>DAAQPARRAVRSSRHHHHHHGSATCAVYGDGHYLTFDGQSYSFNGDCEYTLVQNHCGGKDSTQDSFRVVTENVPCGTTGTTCSKAIKIFLGGFELKLSHGKVEVIGTDESQEVPYTIQQMGIYLVVDTDIGLVLLWDKKTSIFINLSPEFKGRVCGLCGNFDDIAVNDFATRSRSVVGDVLEFGNSWKLSPSCPDALAPKDPCTANPFRKSWAQKQCSILHGPTFAACHAHVEPARYYEACVNDACACDSGGDCECFCTAVAAYAQACHEVGLCVSWRTPSICPLFCDYYNPEGQCEWHYQPCGVPCLRTCRNPRGDCLRDVRGLEGCYPKCPPEAPIFDEDKMQCVATCPTPPLPPRCHVHGKSYRPGAVVPSDKNCQSCLCTERGVECTYKAEACVCTYNGQRFHPGDVIYHTTDGTGGCISARCGANGTIERRVYPCSPTTPVPPTTFSFSTPPLVVSSTHTPSNGPSSAHTGPPSSAWPTTAGTDDDDKTSEQKLISEEDLSRKLTR[4x]

The two gel-forming mucins MUC5AC and MUC5B constitute the main structural components of the mucus protecting the underlying epithelia in the respiratory system. The VWD assemblies are formed by the VWD domain, C8, trypsin inhibitor like (TIL) and E domains, except the VWD’ domain that only has the TIL and E domains. We determined the cryoEM structures of the wild type D3 assembly of the human MUC5AC mucin and the structural single nucleotide polymorphisms (SNP) variants Arg996Gln and Arg1201Trp that affect intermolecular interactions. The D3 assembly forms covalent dimers that can appear in two alternative conformations, open and closed, where the closed conformation dimers interact through an arginine-rich loop in the TIL3 domain to form tetramers.

Similarly, the structure of the tetrameric 6xHis-MUC5AC-D3 Arg996Gln assembly was solved at low resolution (6–7 Å), not enough to reveal the molecular mechanism of the non-covalent oligomerization. Surprisingly, the 6xHis-MUC5AC-D3 Arg996Gln adopts another conformation not observed in the other variants as the protein forms ring shape octamers. The His-tagged Arg996Gln mutant showed a high proportion of octameric particles in cryoEM that were essential for solving the high-resolution structure of the non-covalent interaction. Particle subtraction followed by local refinement let us solve the structure of a tetramer forming part of the octamer at 3.69 Å resolution. The MUC5AC-D3 non-covalent tetramer interaction is driven by the TIL3 domain and involves an interface area of 385.4 Å2. The interaction between the MUC5AC-TIL3 domains occurs in the arginine-rich loop β1-β2 stabilized by a disulfide bond between Cys1185-Cys1196. Intermolecular salt bridges and hydrogen bonds are formed between lateral chains of Asp1199-chainB (Asp1199B) and Arg1198-chainD (Arg1198D), and between Arg1198B lateral chain and the main chain of Arg1193D and Asp1195D, Arg1193D and Cys1185B, and between Arg1198D and Leu1197B and Arg1198B. The comparison between the tetrameric MUC5AC-D3 Arg996Gln assembly and the free closed conformation dimer shows significant differences only in the TIL3 domain region. While the tetramer chain D shows only minor deviations, the TIL3 loop β1-β2 in chain B changes its relative position with C8-3 and VWD3 domains allowing the interaction with chain D. No interactions between the His-tag of one monomer and the core of the other one were observed, just His-tag–His-tag interactions, supporting that it is an unspecific interaction that stabilizes the TIL3-TIL3 interface.Chalcone synthase (CHS) and chalcone isomerase (CHI) catalyze the first two committed steps of the flavonoid pathway that plays a pivotal role in the growth and reproduction of land plants, including UV protection, pigmentation, symbiotic nitrogen fixation, and pathogen resistance. Based on the obtained X-ray crystal structures of CHS, CHI, and chalcone isomerase-like protein (CHIL) from the same monocotyledon, Panicum virgatum, along with the results of the steady-state kinetics, spectroscopic/thermodynamic analyses, intermolecular interactions, and their effect on each catalytic step are proposed. The production of these value-added products also offers the prospect of increasing the value of the crop, especially because many of these compounds are soluble and readily extracted. This study characterized the enzymes involved in the first two committed steps of the flavonoid pathway, CHS and CHI, and the non-catalytic protein CHIL. Through crystal structure, molecular docking, mutagenesis, kinetic analyses, ITC, and FRET analysis, our study provides evidence supporting a revised catalytic reaction mechanism for monocot CHS and CHI and identified an intermolecular interaction of CHS with both CHI and CHIL in a non-competitive manner.

The electron densities corresponding to the residues from 6 to 21 and from 26 to 219 among each of the 223 residues in the native PvCHIL molecule were resolved. The overall secondary structure was composed of eight β-sheets and seven α-helices. The structure of PvCHIL was very similar to that of PvCHI in terms of both the number of secondary structural elements and the overall three-dimensional structure with a backbone RMSD of 1.21 Å. The area of the largest structural differences between PvCHI and PvCHIL was located at the residues corresponding to the ligand-binding pockets of CHI. However, the corresponding primary sequence for those secondary structural features is not conserved, as the active site is replaced in PvCHIL with the following residues: Arg-35 (Thr-37), Thr-47 (Asn-49), Asn-113 (Ser-115), Ser-190 (Trp-193) with Tyr-106 (Tyr-108) as the only conserved active site residue. Close inspection of the results indicated that the PvCHIL utilized its unique protruding loop between β3a and β3b to bind near the homodimer interface of PvCHS. The interaction between PvCHS and PvCHIL was endothermic with ΔH of 31.88 kcal mol−1, ΔS of 127 cal mol−1 deg−1, and Kd of 76.3 µM. In the presence of naringenin and naringenin chalcone, the Kd was 7.46 µM and 170.35 µM, respectively, indicating that in the presence of naringenin, affinity between PvCHIL and PvCHS is increased, whereas affinity between them is decreased in the presence of naringenin chalcone. As previously observed in snapdragon (Antirrhinum majus) CHS, promiscuity of PvCHS was rectified by PvCHIL, yielding much less CTAL and BNY.

>MGSETETVTVEGIPFPAEITFTAGGNPAVSLVGNGITDIEIHFLQIKYNAIGIYLHSNDVLLDHLHGWKGKSADELLGDDSFFQALVAAPVEKLFRVVVIKEIKGSQYGVQLESSVRDRLVAADKYDDDEEEALEKITDFFQAKYFKPGSVITFHFPATSAAGAVEISFATEGKDAAKMKVENENVARMIQKWYLGGDSAVSPTTVRSMADRFAALLSAASEF[2x]> SMIMEIPAIKALSRYAQWVIWKKERDTKIPYNPNNGKKASSTDPLAWGDIDEAQ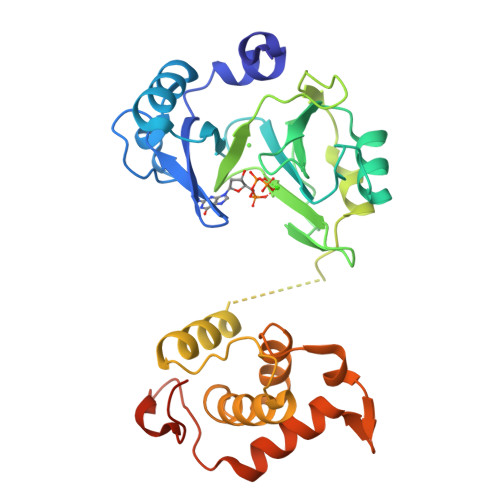AGLVRYGANGLGFVLTKSDPFVFIDLDHVLDENKRVKCEWARQLLKEIKSYTEISPSGDGLHVVVSGKLPDYIKHKTKFDDGSALEVYESGRYMTITGEVFDGRDDIKELDLSILGEFAEHKIETKNAPVQIESATTLDDEAIIDLMKRKGQWPDAPKDGDDWSSLDMSFANRLAFWCGKDIERMDRIFRQSPLMRQKWDRPTAGSTYGRITLKKACDFVDSVYDPALRNESDCPFEPYNEEGGPRNDKEEK3-[(2~{S},3~{R})-2-carboxypyrrolidin-3-yl]propyl-$l^{3}-oxidanyl-bis(oxidanyl)boranuide 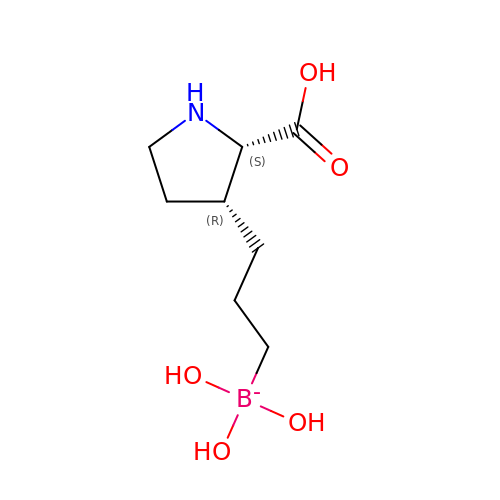| C8 H17 B N O5 | SKGPQQUJOITTRF-RQJHMYQMSA-N> SVPQARKASLARFLEKRKE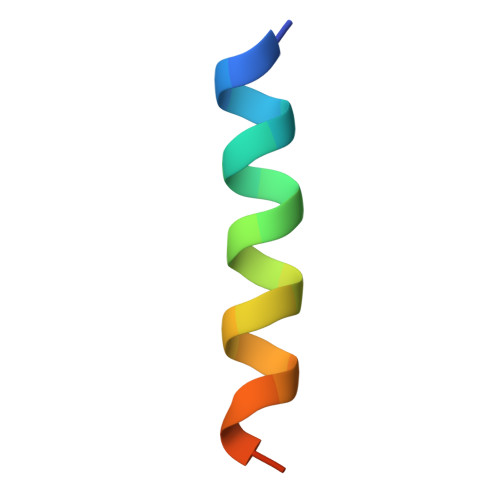RLM>[2x]MSTAKSFPMAQLSTRAQYSRMQREFVQLQRQENPRNINFTTSLKNRHKNRYLDILANEETIYPPVLKAVGAQPGRYPYINGNLID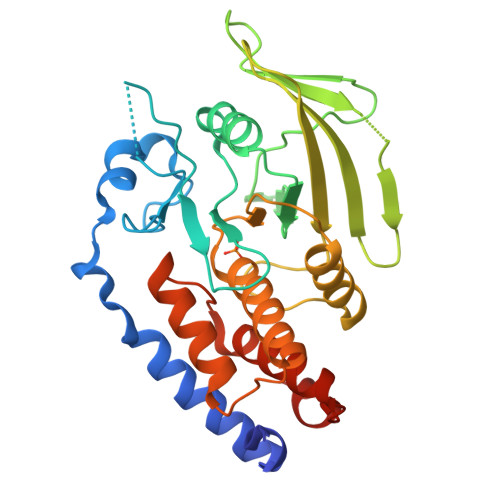LDLPHTFVACQAPVPQGVPDFLETLSEKKVDLVVMLTKLREGGVLKAERYWPEEEEDSLSFPESGHDAIKVTRDAEASYEVDAELDIVRRPLVIHVPGKPMHRVLQVQYVGWPDHGVPESAASFDELLSVIKNCVTTSPILVHCSAGIGRTGTLIGAYAALLHIERGILTDSTVYSIVAAMKQKRFGMVQRLEQYAVIYMTVLGRLGVDISGLVSTLNLKA>DNDPLVVNTDKGRIRGITVDAPSGKKVDVWLGIPYAQPPVGPLRFRHPRPAEKWTGVLNTTTPPNSCVQIVDTVFGDFPGATMWNPNTPLSEDCLYINVVAPRPRPKNAAVMLWIFGGGFYSGTATLDVYDHRALASEENVIVVSLQYRVASLGFLFLGTPEAPGNAGLFDQNLALRWVRDNIHRFGGDPSRVTLFGESAGAVSVSLHLLSALSRDLFQRAILQSGSPTAPWALVSREEATLRALRLAEAVGCPHEPSKLSDAVECLRGKDPHVLVNNEWGTLGICEFPFVPVVDGAFLDETPQRSLASGRFKKTEILTGSNTEEGYYFIIYYLTELLRKEEGVTVTREEFLQAVRELNPYVNGAARQAIVFEYTDWTEPDNPNSNRDALDKMVG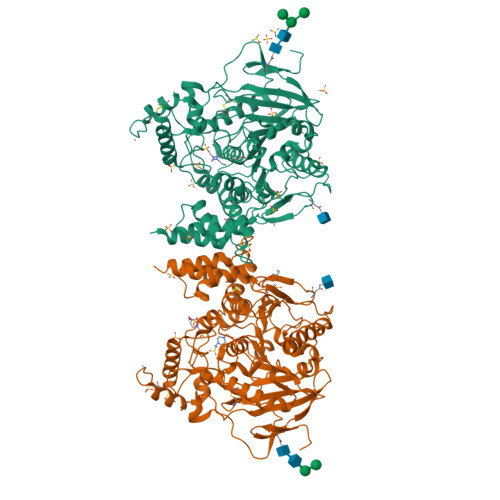DYHFTCNVNEFAQRYAEEGNNVYMYLYTHRSKGNPWPRWTGVMHGDEINYVFGEPLNPTLGYTEDEKDFSRKIMRYWSNFAKTGNPNPNTASSEFPEWPKHTAHGRHYLELGLNTSFVGRGPRLRQCAFWKKYLPQLVAATSNLPGPAPPSEPCESSAFFYRPDLIVLLVSLLTATVRFIQ[2x]>MGAAILPDLGTEILIPVCAVIGIAFALFQWLLVSKVKLSAVRDASPNAAAKNGYNDYLIEEEEGINDHNVVVKCAEIQNAISEGATSFLFTEYKYVGIFMVAFAILIFLFLGSVEGFSTSPQACSYDKTKTCKPALATAIFSTVSFLLGGVTSLVSGFLGMKIATYANARTTLEARKGVGKAFITAFRSGAVMGFLLAANGLLVLYIAINLFKIYYGDDWGGLFEAITGYGLGGSSMALFGRVGGGIYTKAADVGADLVGKVERNIPEDDPRNPAVIADNVGDNVGDIAGMGSDLFGSYAESSCAALVVASISSFGLNHELTAMLYPLIVSSVGILVCLLTTLFATDFFEIKAVKEIEPALKKQLVISTVLMTIGVAVVSFVALPTSFTIFN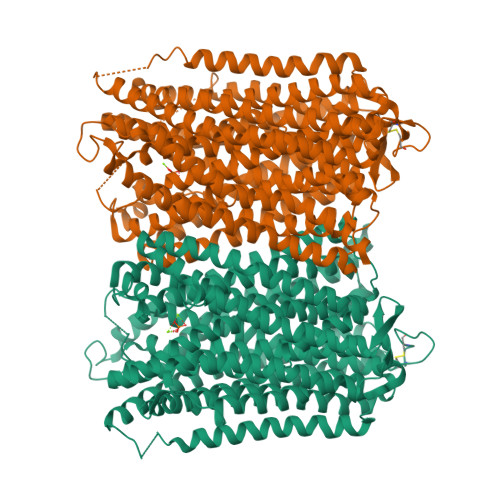FGVQKDVKSWQLFLCVAVGLWAGLIIGFVTEYYTSNAYSPVQDVADSCRTGAATNVIFGLALGYKSVIIPIFAIAISIFVSFTFAAMYGIAVAALGMLSTIATGLAIDAYGPISDNAGGIAEMAGMSHRIRERTDALDAAGNTTAAIGKGFAIGSAALVSLALFGAFVSRASITTVDVLTPKVFIGLIVGAMLPYWFSAMTMKSVGSAALKMVEEVRRQFNTIPGLMEGTAKPDYATCVKISTDASIKEMIPPGALVMLTPLVVGILFGVETLSGVLAGSLVSGVQIAISASNTGGAWDNAKKYIEAGASEHARSLGPKGSDCHKAAVIGDTIGDPLKDTSGPSLNILIKLMAVESLVFAPFFATHGGLLFKIFSSHHHHHH[4x]>MPRKKDQVTKNDDGNQTSDVQTQDFKTAVQPDTNTAQLIKTYSNPKQRGDKGEIIYDGGLSSKLADVVDKTTEPHNADGAVKDGRIAPVKLDLEKQKLDKLKLFETSPFDPLTIKNNQDVVDKLYATQSSSIQEVVPTKTFATELQFGVTSEDMAKIYGAVAAVSKNVNSSVTYEVKRGTHELIKVPTIPHNLVLIQSDNGKHALIKEDLGQWPVETGISLVNQAGVFAVQLANKLGIDKPFVLDAGSNYFTDTSFIDTRKYCTDGLSPREIQKALNRQRAYYDRPELTISENKTLLSQSIIYPDADGNDVSIIFSGAMSHAIFTYAQSQWNKNIIKLDDYIREITLTVPKQYRPRRFKEIEHTHGYVYRELNQGSLLPLVDANLKESSSYYFKKLMSSISNVPVDARTLQSATAALAADTGQAVNRAQHVSMLTNRLTTANAPTVRAITVLTCMFKQFRIGMTYALDPNIMDVAAATCMLLFRPAQSISDEQYRYCLQTMAVFLTNTTYDIVNNDTIDVLKMKLRNQGWPFVERYNAVEIDMSVEPLRSPGQVGRYYNPFNIDPLTKKHVEDRLEEFINQVQVGRFRNASGNAVGTTLAAFLRACRDKTSANWRGYSVLVSRYRSLIPNELFESLRNISGEYNINPQDEHSFFFALAQINADDEFIGAIDKESAEYLDEYATLARDISNSLTLVKAAFGPLERTSGSIINHANNLNKVINHVFADKPLISETMLKILTIDGTTGKDGYRNWLDKLVGHNYPVYVEPVVNIMNFISARFVADSSYFGYTNEIMIMPNHINVPVDDRFGFRDSPFCTSLPRTIMGNDVRRISYNVFSMMEDIDDVISEGFILYDAYFNFSYDIMTTDGVTRLKEDILIVTDTGNDIKPIHFYIYFENRNDKKLRYESKMNVSYRLYIKTPACLLPLSDYMRAQHDYVSPSSSRVYIKDPAVVYTRS[11x];> MDVQEQFEGYLREEVDLLNKFEDSHFKQLEIFYTKSQTDHVINKDKLQFNALPFHTTLYKEINGKRVRLGTLLNWTKAERLDTIRHESMIKDERLRRLIDFDYGWIDYAVVLQRYLDEGNTIESANILQFDGDFVNNIKHPTQKNNFLDIKVIKECETYILMKDDNGIRDPDILRAWELNSIPEVIELDVDGETKKFNLRKEMIKRIQDEAPVYFFCNPYRYAVANLDPNIPEVRLWLEYFIGSEDFFGFNGPNVIVSKSLLAAKRFEVVVNHLRKVAAFELDVESKEVMNEWIKYIMIDPVYRSYKNRGAFGNLNQHVFARTKSEGLSWSLIDIGTTNFELKPTKKVAGSYVNKFNLVDDVLVEESLKDLRNEGLHKMADVTRRMIDADITPENVKKGKLNRLALSYCGYTGSHSATAMVKQFNGTKDLDPNCDPMFVDIVKDNMRVYMQEGLQKYPQGSRKSNRLDILFKGGTSSASSTNEHAVVNGRFRYRSELYRERDVNSSTVFKTATPGQYRVVKKISAKLKSKNANIVTHPMNFINFKVDDLDIVVNAGSRLVRGTRAKRIITPNYGTIYAASLMTVLPAVRLLSSRASNMGALSTQGRIGTTYHGALPHDVMAPQLAVTSSDDVSKICVAKDFGQFDTSQWGQISKAHADGVRSMKAHYSMGHDTLVDLDLNDASFADLLEVTAMSYERPLKYKMNGLVCESAGVKSGELTTQTRNTTTNISHSTVALDDYNNRAYRLNLPKLELVTDNKVGDDSVEVLRVVDGSPLTPEIAKLYVNCMQDHADKNHLEISAKRTIVGNNVAEHIKIWVFKGYLALDVFLDSVTSEKNSFSNLNYLEQVNILYDMAMTLM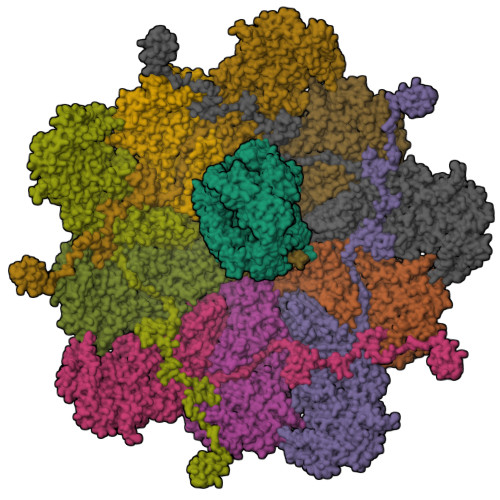IRYCSVQACMTQFCNDMKLLNGIRAGNYTFIPTPKIICAYGTPEICLRAPEIRSFGRYLPIDEDEYSVLNDLVASLSTNKPKMDFVAQMFEQNGNQVHGIWLDHFKRKNDVNPDGGGIHISEGLKRLMPEYCERHLNELVYKTLDDKVIRDYTSDIIITNICKGKLSKAPKLAFFANFYLSLTGFNGVDSPYLTADEGVKNVHRVIGLSYRNTLSTSPTANVDRILRNNPGSAPAYLTGNDILGVLSDYPYQNWRTVVELLDITEPSATAIIEVATNQMHAYLADKDLNTANLFDNTSRTYDISDRTYPKFVNITSNLSNSNRRGFQLEAMKHIIYMARRGIATLANTHPSKIGNTVYYDY> TQELGNANFENFIGATEGFSEIAYQFTSHILTLGYAVMLAGLLYFILTIKNVDKKFQMSNILSAVVMVSAFLLLYAQAQNWTSSFTFNEEVGRYFLDPSGDLFNNGYRYLNWLINVPMLLFQILFVVSLTTSKFSSVRNQFWFSGAMMIIT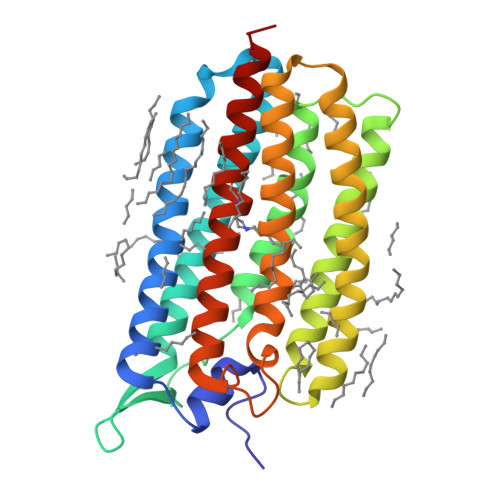GYIGQFYEVSNLTAFLVWGAISSAFFFHILWVMKKVINEGKEGISPAGQKILSNIWILFLISWTLYPGAYLMPYLTGVDGFLYSEDGVMARQLVYTIADVSSKVIYGVLLGNLAITLSKNKEL3-(decyloxy)-5-(3,5-difluorophenyl)-1-(2,2-diphosphonoethyl)pyridinium 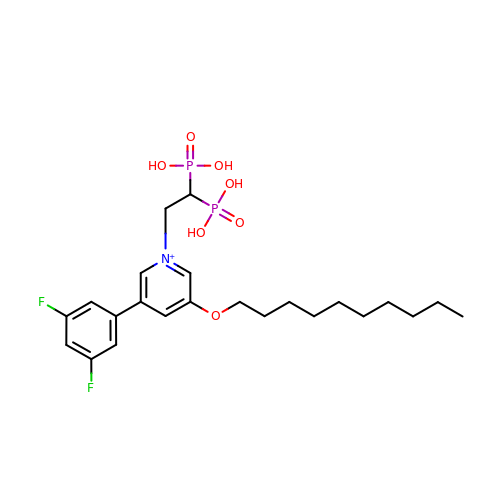| C23 H34 F2 N O7 P2 | JONDYIHZOFRLBH-UHFFFAOYSA-O>[2x]MSTEIKTQVVVLGAGPAGYSAAFRCADLGLETVIVERYNTLGGVCLNVGCIPSKALLHVAKVIEEAKALAEHGIVFGEPKTDIDKIRTWKEKVINQLTGGLAGMAKGRKVKVVNGLGKFTGANTLEVEGENGKTVINFDNAIIAAGSRPIQLPFIPHEDPRIWDSTDALELKEVPERLLVMGGGIIGLEMGTVYHALGSQIDVVEMFDQVIPAADKDIVKVFTKRISKKFNLMLETKVTAVEAKE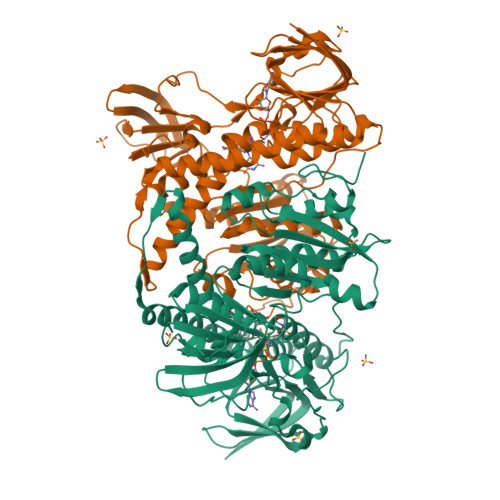DGIYVTMEGKKAPAEPQRYDAVLVAIGRVPNGKNLDAGKAGVEVDDRGFIRVDKQLRTNVPHIFAIGDIVGQPMLAHKGVHEGHVAAEVIAGKKHYFDPKVIPSIAYTEPEVAWVGLTEKEAKEKGISYETATFPWAASGRAIASDCADGMTKLIFDKESHRVIGGAIVGTNGGELLGEIGLAIEMGCDAEDIALTIHAHPTLHESVGLAAEVFEGSITDLPNPKAKKK>MRPITCSFDPVGISFQTESKQENFEFLREAISRSVPGLENCNVFDPRSLGVPWPTSFPAAAQSKYWKDAEEAAAELMDQIVAAAPGEQGSLPAELAVSDKKAAKRRELLDTSVSAPMNMFPAANAPRARIMAKAALLIFMHDDVCEYQSVQSTIIDSALADTSTPNGKGADILWQNRIFKEFSEETNREDPVVGPQFLQGILNWVEHTRKALPASMTFRSFNEYIDYRIGDFAVDFCDAAILLTCEIFLTPADMEPLRKLHRLYMTHFSLTNDLYSFNKEVVAEQETGSAVINAVRVLEQLVDTSTRSAKVLLRAFLWDLELQIHDE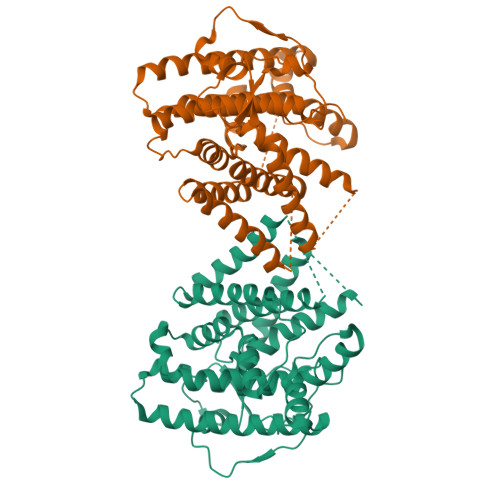LTRLKGTDLTPSQWRFARGMVEVCAGNIFYSATCLRYAKPGLRGI[4x]IL-1β is a key cytokine at the interface of innate and adaptive immunity. IL-1β is produced as a 269 amino acid precursor protein, which is cleaved by molecular platforms known as inflammasomes that assemble under pro-inflammatory conditions, leading to extracellular release of its C-terminal 153 amino acid-containing mature form. The binding of mature IL-1β to its cognate receptor IL-1R1 on nearby cells and subsequent formation of a ternary signaling complex with IL-1RAcP triggers a pro-inflammatory response with the production of inflammatory mediators, such as IL-64. hIL-1β belongs to a family of 11 cytokines that all share the same β-trefoil-fold structure despite divergent amino-acid sequences (IL-1α, IL-1Ra, IL-18, IL-33, IL-36α, IL-36β, IL-36γ, IL-36Ra, IL-37, IL-38).

The crystal structure of the hIL-1β/(S)-2 complex shows the binding of the ligand to a cryptic pocket formed upon displacement of loop β4–5 by up to 11 Å from its position in mature hIL-1β. The X-ray structure shows a short hydrogen bond formed between the main chain carbonyl oxygens of Lys93 and Met95 and the phenol hydroxyl (2.5 Å) and the indolinone lactam nitrogen (2.8 Å) of the ligand, respectively. These two polar interactions anchor the ligand in the cryptic pocket and are thus critical interactions between the ligand and the cytokine, as shown by the lack of binding of the methylated analogs 4 and 5. The indolinone moiety (ring A, ring B) binds deep into the hydrophobic core of the cryptic pocket facing the side chains of Val3, Val47, Pro57, Met95, and Val100. The pyrazole group engages in a hydrogen-bonded interaction with the side-chain of Glu50, which is part of the loop β4–5. The para benzoic acid group is H-bonded to Asn102 Nδ2 and makes water-mediated interactions with Lys55 Nζ, Lys97 Nζ, and the main chain carbonyl oxygen of Ala115. The ortho benzoic acid group is H-bonded to Lys97 Nζ and forms a long ionic interaction with Lys94 in one of the two complexes making up the asymmetric unit of the crystal. The binding of (S)-2 to hIL-1β did not perturb the conformation of residues at site A. In contrast, in the ligand-bound state, loop β4–5 adopts a conformation that is incompatible with the receptor-bound state of the cytokine at site B, which thus forms the structural basis for the antagonistic activity of (S)-2 and its analogs. Intriguingly, the minor form involves residues Val47, Gln48, Lys92, and Lys94, which are all critically involved in the formation of the binding site of compound (S)-2.

>APVRSLNCTLRDSQQKSLVMSGPYELKALHLQGQDMEQQVVFSMSFVQGEESNDKIPVALGLKEKNLYLSCVLKDDKPTLQLESVDPKNYPKKKMEKRFVFNKIEINNKLEFESAQFPNWYISTSQAENMPVFLGGTKGGQDITDFTMQFVSS[2x]> VGSLNCIVAVSQNMGIGKNGDLPWPPLRNESRYFQRMTTTSSVEGKQNLVIMGKKTWFSIPEKNRPLKGRINLVLSRELKEPPQGAHFLSRSLDDALKLTEQPELANKVDMV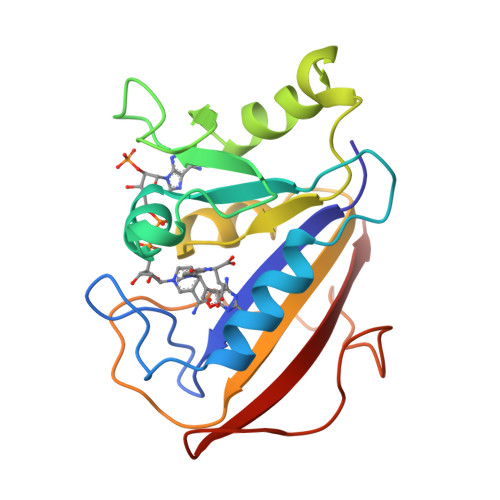WIVGGSSVYKEAMNHPGHLKLFVTRIMQDFESDTFFPEIDLEKYKLLPEYPGVLSDVQEEKGIKYKFEVYEKND>[2x]MNLPTAQEVQGLMARFIELVDVGDIEAIVQMFADDATVEDPFGQPPIHGREQIAAFYRQGLGGGKVRACLTGPVRASHNGCGAMPFRVEMVWNGQPCALDVIDVMRFDEHGRIQTMQ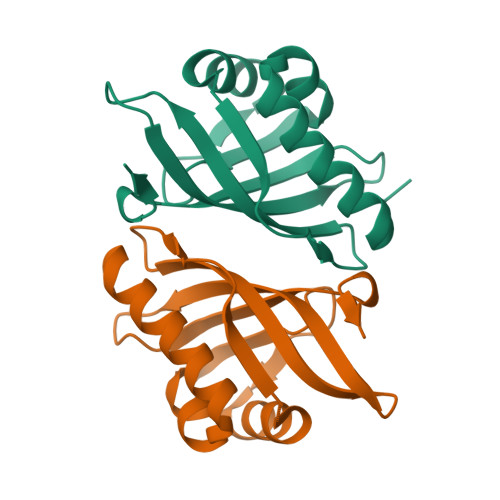AYWSEVNLSVREPQ> AILS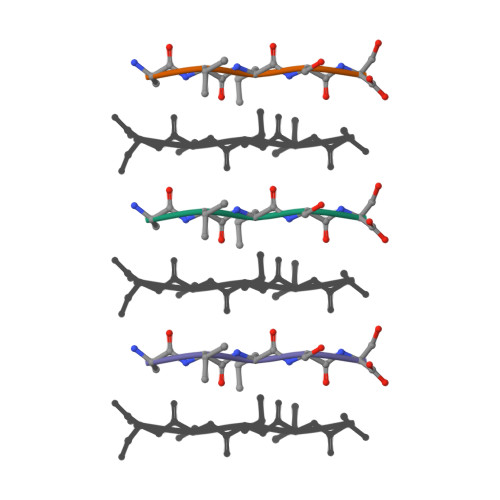S The bacterial tight adherence pilus system (TadPS) assembles surface pili essential for adhesion and colonisation in many human pathogens. Pilus dynamics are powered by the ATPase CpaF (TadA), which drives extension and retraction cycles in Caulobacter crescentus through an unknown mechanism. We show that CpaF assembles into a hexamer with C2 symmetry in different nucleotide states. Nucleotide cycling occurs through an intra-subunit clamp-like mechanism that promotes sequential conformational changes between subunits.

To understand how different nucleotide states might regulate CpaF assembly and conformation, the structure of CpaF was determined by cryo-EM in the presence of ADP and Mg2+. CpaF incubated with ADP yielded our highest quality map at 3.1 Å resolution overall facilitating a build of the NTD2 and CTD with excellent sidechain detail for all subunits. Henceforth, this CpaF structure obtained in the presence of ADP is termed CpaFADP. CpaFADP formed a C2 symmetric hexamer with dimensions and subunit packing similar to CpaFAMPPNP. However, ADP/Mg2+ was now bound in each nucleotide-binding pocket. In CpaFADP, the map around the nucleotide binding pocket was now fully ordered with the P-loop well resolved. Crucially, HIS box residue H382 was turned away from the nucleotide with P-loop K287 fully engaging the β-phosphate just like in CpaFAMPPNP open state. Moreover, superposition of subunits for CpaFADP open’ state with CpaFAMPPNP open state, including their interfaced CTDn+1, revealed remarkable similarity with RMSD Cα = 1.0 Å. Broadly, this means that when ADP/Mg2+ is bound to CpaFADP in the open state, then the nucleotide binding pocket of the open’ state subunit resides in a conformation similar to the open state of CpaFAMPPNP. This finding suggests a model where the CpaFADP open’ state has the appropriate conformation and geometry of key residues to support AMPPNP (or ATP) binding when ADP/Mg2+ is bound in the open state subunit. As the nucleotide binding pockets are solvent accessible in both these states, the CpaFADP structure is consistent with the nucleotide switch model where ATP and ADP binding in the open’ and open states, respectively, would potentiate counter-clockwise motion.

>[6x]DYYHATKTTIFNALLNTIDLSQLAQLDLKQAGEEIRDIVAELVAIKNVSMSVAEQEHLVQDIINDVLGYGPLEPLLARDDIADIMVNGAHRVFIEVGGKVQLTNVRFRDNLQLMNICQRIVSQVGRRVDESSPICDARLPDGSRVNVIAPPLALDGPTLTIRKFKKDKLTMKNLVEFASISPEGARVLGVIGACRCNLVISGGTGSGKTTLLNTMTAFIDPTERVVTCEDAAELQLQQPHVVRLETRPPNLEGSGAVTMRDLVKNCLRMRPERIIVGEVRGPEAFDLLQAMNTGHDGSMGTLHANSPREAISRIESMITMGGYGLPSKTIKEMIVGSVDVIIQAARLRDGSRRITHITEVVGLEGDVIVTQDLFVYEITGEDEHGKVVGKHRSTGIARPRFWDRARYYGLERELAEALDAAEAL> MTIKNVICDIDGVLMHDNVAVPGAAEFLHGIMDKGLPLVLLTNYPSQTGQDLANRFATAGVDVPDSVFYTSAMATADFLRRQEGKKAYVVGEGALIHELYKAGFTITDVNPDFVIVGETRSYNWDMMHKAAYFVANGARFIATNPDTHGRGFYPACGALCAGIEKISGRKPFYVGKPSPWIIRAALNKMQAHSEETVIVGDNLRTDILAGFQAG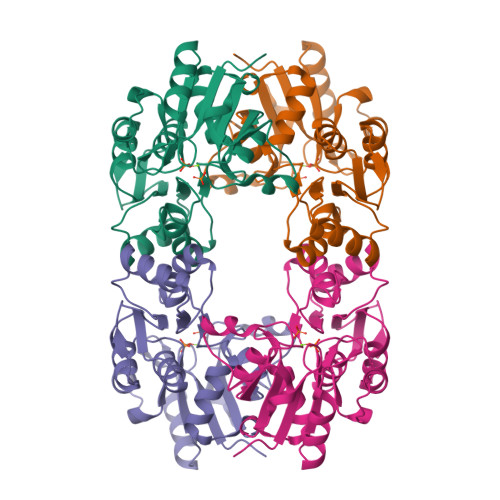LETILVLSGVSSLDDIDSMPFRPSWIYPSVAEIDVI> MPKHGKRYRALLEKVDPNKIYTIDEAAHLVKELATAKFDETVEVHAKLGIDPRRSDQNVRGTVSLPHGLGKQVRVLAIAKGEKIKEAEEAGADYVGGEEIIQKILDGWMDFDAVVATPDVMGAVGSKLGRILGPRGLLPNPKAGTVGFNIGEIIREIKAGR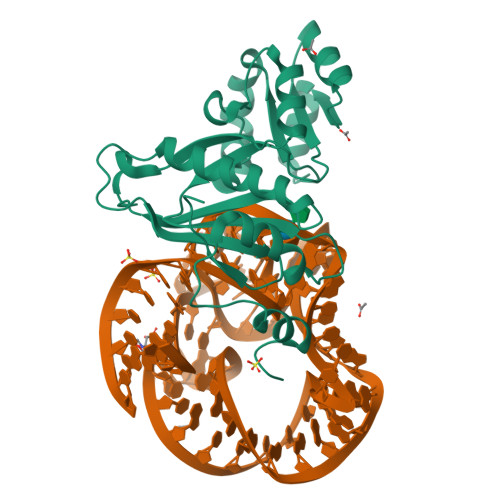IEFRNDKTGAIHAPVGKASFPPEKLADNIRAFIRALEAHKPEGAKGTFLRSVYVTTTLGPSVRINPHS>GSHMSTLRLLISDSYDPWFNLAVAECIFRQMPATQRVLFLWRNADTVVIGRAQNPWKECNTRRMEEDNVRLARRSSGGGAVFHDLGNTCFTFMAGKPEYDKTISTSIVLNALNALGVSAEASGRNDLVVKTVEGDRKVSGSAYRETKDRGAHGGTLLLNADLSRLANYLNPDKKKLAAKGITSVRSRVTNLTELLPGITHEQVCEAITEAFFAHYGERVEAEIISPNKTPDLPNFAETFARQSSWEWNFGQAPAFSHLLDERFTWGGVELHFDVEKGHITRAQVFTDSL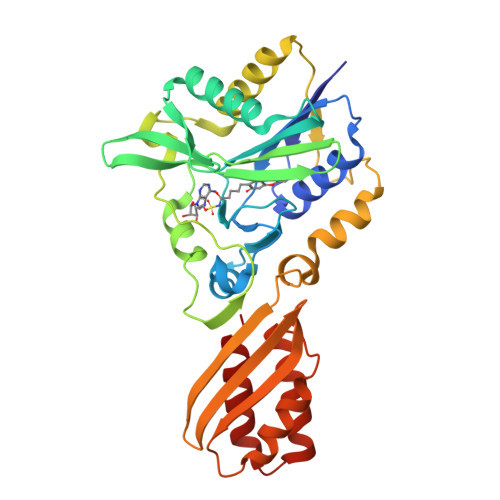NPAPLEALAGRLQGCLYRADMLQQECEALLVDFPEQEKELRELSAWMAGAVR[4x]> GPLGSPEFDCHLSDMLQQLHSVNASKPSERGLVRQEEAEDPACIPIFWVSKWVDYSDKYGLGYQLCDNSVGVLFNDSTRLILYNDGDSLQYIERDGTESYLTVSSHPNSLMKKITLLKYFRNYMSEHLLKAGANITPREGDELARLPYLRTWFRTRSAIILHLSNGSVQINFFQDHTKLILCPLMAAVTYIDEKRDFRTYRLSLLEEYGCCKELASRLRYARTMVDKLLSSR;> XFMPPPMSSMX

We examined the crystal-packing interactions formed by the polo-box domain (PBD) of polo-like kinase 1 (Plk1), a validated anti-cancer target, whose phosphorylation-dependent protein–protein interactions are crucial for successful progression of the cell through mitosis. We have observed an unreported binding site in a number of crystal structures of the PBD, which is formed by the rearrangement of surface residues involved in crystal packing. This site is located close to the phosphopeptide-binding groove, making it potentially accessible for phosphorylated proteins binding to the PBD. The new binding site consists of seven residues: Val415, Leu478, and Phe482 form the bottom of the pocket whilst Tyr417, Tyr421, Tyr481, and Tyr485 form the sides of the pocket.

Only 2 out of 631 proteins—TCERG1 (transcription elongation regulator 1) and PBIP1 (polo-box interacting protein 1)—met our search criterion. Interaction between TCERG1 and PBD has not been characterized in detail before. Interestingly both proteins contain the sequence FXP, resembling the sequence involved in one of the observed crystal contacts. Pro103TCERG1 in TCERG1 occupies the place of Leu75PBIP1 in PBIP1 and imposes a conformational restraint that prevents the FMP motif from turning into the hydrophobic pocket, which is occupied by polyethylene glycol used in the crystallization buffer.> MSFINYSSREINCKIVYYGPGLCGKTTNLQYIYNKTAAETKGKLISLSTETDRTLFFDFLPLSLGEIRGFKTRFHLYTVPGQVFYDASRKLILKGVDGVVFVADSQIERMEANMESLENLRINLAEQGYDLNKIPYVIQYNKRDLPNAVTVEEMRKALNHRNIPEYQAVAPTGVGVFDTLKAVAKLVLTELKKGGHHHHHH

A hallmark of all motile M. xanthus cells is the accumulation of MglA-GTP at the leading pole where it activates motility, while MglA-GDP is found diffusely in the cytosol. This localization pattern arises due to the GAP activity of MglB, which is located at the lagging pole where it inactivates MglA-GTP and depletes it from this pole. The ability of MglA to hydrolyze GTP is essential for motility regulation. To gain insight into the structural landscape of M. xanthus MglA, we determined the crystal structures of MglA in different nucleotide states, which uncovered that MglA can adopt three conformations: inactive MglA-GDP, active MglA-GTPγS, whose structure had not been determined before, and an unusual conformation combining inactive and active features.

The structure of unbound MglA-GTP is currently unknown, leaving open the question of whether the substantial remodeling at switch 1 and switch 2 is solely due to GTP or is promoted by MglB. Binding of GTPγS induces a twisted three-residue register shift of switch 1 and remodels switch 2 to create space for the γ-phosphate, as seen in MglA in the T. thermophilus MglA-MglB complex12. The shift of switch 1 results in the elongation of the arginine finger loop (residues 44−58), but Arg53 remains outside the nucleotide-binding site. Displacement of switch 2 also allows Mg2+ to bind with an incomplete coordination that lacks the conserved Mg2+-binding threonine (Thr54) located in the arginine finger loop. Accordingly, the MglB-sensitive MglA-GTP species is likely represented by the MglA-GTPγS structure, in which both switch regions are in active conformations similar to those seen in the MglA/MglB complex (this study, 12).>[2x]MVGSLNCIVAVSQNMGIGKNGDLPWPPLRNEFRYFQRMTTTSSVEGKQNLVIMGKKTWFSIPEKNRPLKGRINLVLSRELKEPPQGAHFLSRSLDDA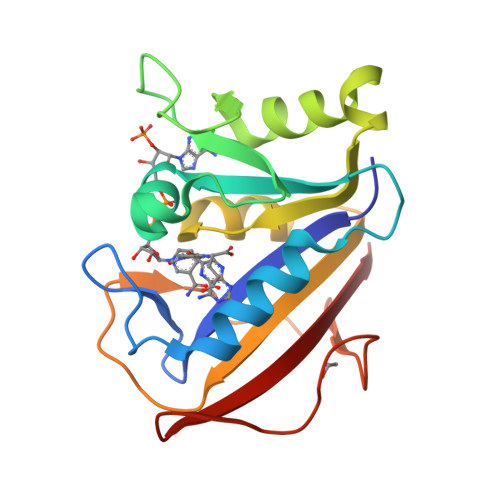LKLTEQPELANKVDMVWIVGGSSVYKEAMNHPGHLKLFVTRIMQDFESDTFFPEIDLEKYKLLPEYPGVLSDVQEEKGIKYKFEVYEKND> MKSSHHHHHHENLYFQSNAKQALLWRDSETFILTSIELYNWGGFQGYHRAEIDPSGTAVIGPTGSGKTTLVDALMTLLCANPRYNLASTGGHESDRDLVSYVRGVTGPGDGGVEQSHIARQGKTVTAIAATLERDGAQVRLGAVLWFEGTSSSASDLKKLWLLSESPEQTLEHWLSQHHAGGMRALRQMEKDGMGIWPYPSKKAFLARLRDYFEVGENAFTLLNRAAGLKQLNSIDEIFRELVLDDRSAFERAAEVASSFDDLTDIHRELETARKQQRSLQPVADGWERYRALQEQLQDKQALEGILPVWFAEQGYRLWLAETNRLEKEHKQAELDQAQCRSQLEIQKGVVDQHRQRYLRVGGAGIDQLRGRIADWVRECDKRRLKAEQYQRLAKGLGLADELSAAALEENQQQIAARLEILAQQTTDARQKAFDAGLVQQELNGRLQSLQQERAEVERRPGSNLPGHFHAFRGDLAQELGVDESALPFVAELVQVKPEELAWRGAIERAIGSHRLRILVPQGSSQAALRWVNQRHNRLHVRLLEVKEPSSRPVFFDDGFTRKLTFKEHPYREAVKALLADNDRHCVESTEQLRHTPHAMTAQGLMSGKERFFDKQDQKRLDEDWLTGFDNRDRLAFLAEQIREVNEQLVPAKLALDAAQGDVGQLESQASLLQRIEELQFDDIDRPGAERQLQSLRTQLDTLTRPDSNLAVIKAELDQAEALRESLDQQLQRLIEQCVQLKTQFDQAASATRKAYRGAEKGLSDTQRELAQAHFPILSTDDLGDIDELERKHTRELQGQLKTLGEKLGDQKTELAKRMSDALKADTGALAEVGRELVDVPRYLERLRVLTEEALPEKLKRFLEYLNRSSDDGVTQLLSYIDHEVSMIEERLDDLNSTMQRVDFQPGRYLRLVAKKVIHESLRTLQHAQRQLNSARFIDDEGESHYKALQALVGLLKDACEHSRNQGAKALLDPRFRLEFAVSVIDREGNNLIETRTGSQGGSGGEKEIIASYVLTASLSYALCPDGSSRPLFGTIVLDQAFSRSSHAVAGRIIAALR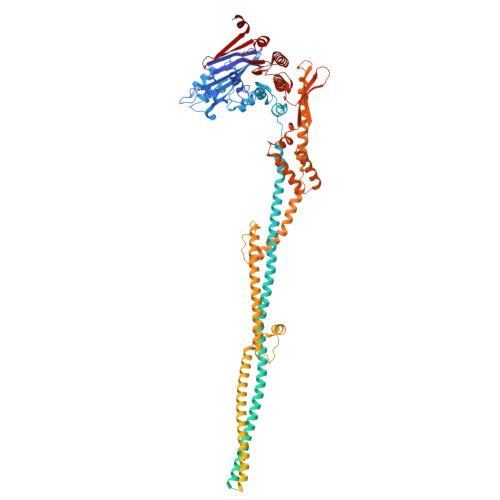EFGLHAVFITPNKEMRLLRHHTRSAVVVHRRGVESSLVSLSWEALDEHHQQRIRAMHEVAH>[2x]MAKKTSSKGKLPPGPFP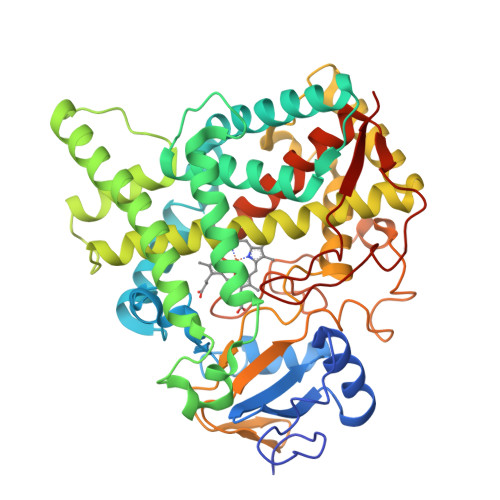YPIVGNMLQLGAQPHETFAKLSKKYGPLMSVHLGSLYTVIVSSPEMAKEIMLKYGTVFSGRTVAQAVHACDHDKISMGFLPIGAEWRDMRKICKEQMFSHQSMEDSQGLRKQKLQQLLDHAHRCSEQGRAIDIREAAFITTLNLMSATLFSMQATEFDSKVTMEFKEIIEGVASIVGVPNFADYFPILRPFDPQGVKRRADVYFGRLLALIEGYLNDRIQSRKANPDAPKKDDFLETLVDILNSNDNKLKTDHLLHLMLDLFVGGSETSTTEIEWIMEELVAHPDKMAKVKAELKSVMGDEKVVDESLMPRLPYLQAVVKESMRLHPPGPLLLPRKAESDQVVNGYLIPKGTQVLINAWAMGRDSTIWNNPDAFQPERFLDNKIDFKGQDYELIPFGSGRRVCPGMPLANRMLHTVTATLVHNFDWKLERPDAPLAEHQGVLFGFAVRRAVPLRIVPYK N-(6-cyano-3-{2-[2-(2,4-dioxo-3,4-dihydropyrimidin-1(2H)-yl)ethoxy]phenoxy}-4-methylnaphthalen-1-yl)-N-methylacetamide 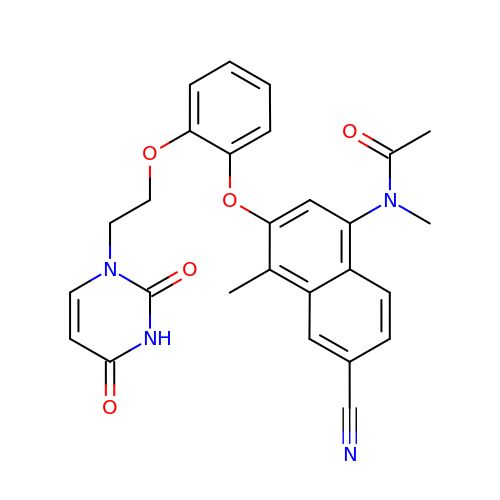| C27 H24 N4 O5 | BUPXJFBLNQOLSS-UHFFFAOYSA-N> HQLQPRRVSFRGEASETLQSPGYDPSRPESFFQQSFQRLSRLGHGSYGEVFKVRSKEDGRLYAVKRSMSPFRGPKDRARKLAEVGSHEKVGQHPCCVRLEQAWEEGGILYLQTELCGPSLQQHCEAWGASLPEAQVWGYLRDTLLALAHLHSQGLVHLDVKPANIFLGPRGRCKLGDFGLLVELGTAGAGEVQEGDPRYMAPELLQGSYGTAADVFSLGLTILEVACNMELPHGGEGWQQLRQGYLPPEFTAGLSSELRSVLVMMLEPDPKLRAT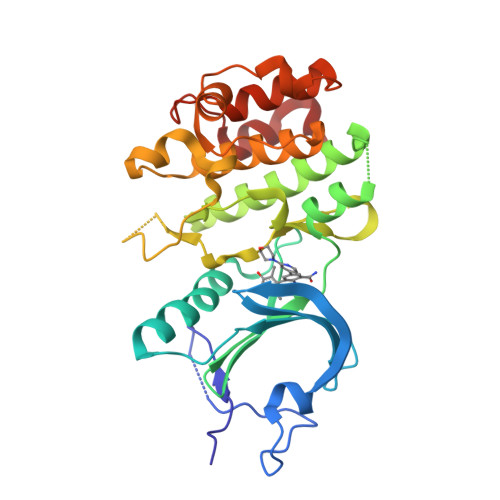AEALLALPVLRQ> VVGGLVALRGAHPYIAALYWGHSFCAGSLIAPCWVLTAAHCLQDRPAPEDLTVVLGQERRNHSCEPCQTLAVRSYRLHEA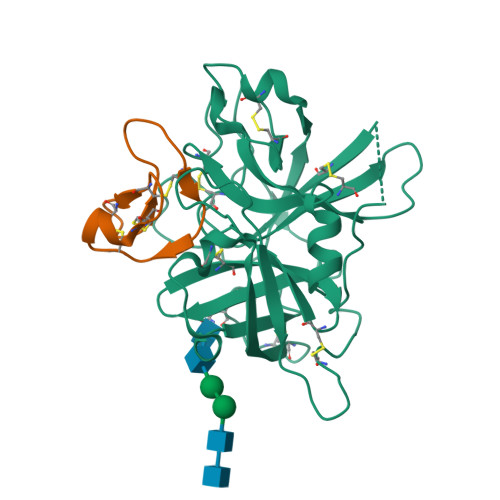FSPVSYQHDLALLRLQEDADGSCALLSPYVQPVCLPSGAARPSETTLCQVAGWGHQFEGAEEYASFLQEAQVPFLSLERCSAPDVHGSSILPGMLCAGFLEGGTDACQGDSGGPLVCEDQAAERRLTLQGIISWGSGCGDRNKPGVYTDVAYYLAWIREHT;> DGGICPRIGRLCRRDSDCPGACICRATRFCGSGY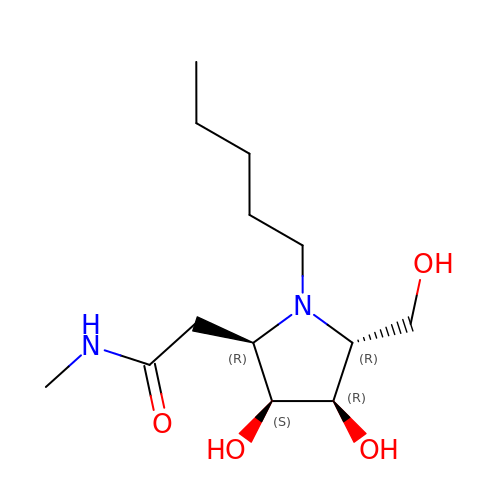2-[(2R,3S,4R,5R)-5-(hydroxymethyl)-3,4-bis(oxidanyl)-1-pentyl-pyrrolidin-2-yl]-N-methyl-ethanamide | C13 H26 N2 O4 | NZYWNYJYZSBEBH-VCDKRKBESA-N> MKFKWDEFFVTGDPLILGAQVSIALSTIAIIFVLTYFKKWKWLWSEWITTVDHKKLGIMYIISAVIMLFRGGVDGLMMRAQLALPNNSFLDSNHYNEIFTTHGTIMIIFMAMPFLIGLINVVVPLQIGARDVAFPYLNNLSFWTFFVGAMLFNISFVIGGSPNAGWTSYMPLASNDMSPGPGENYYLLGLQIAGIGTLMTGINFMVTILKMRTKGMTLMRMPMFTWTTLITMVIIVFAFPVLTVALALLSFDRLFGAHFFTLEAGGMPMLWANLFWIWGHPEVYIVILPAFGIFSEIISSFARKQ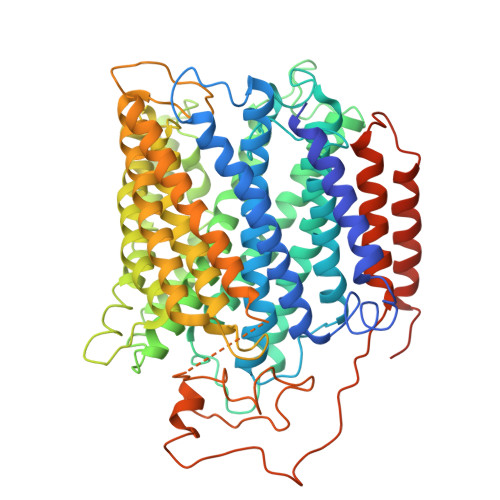LFGYKAMVGSIIAISVLSFLVWTHHFFTMGNSASVNSFFSITTMAISIPTGVKIFNWLFTMYKGRISFTTPMLWALAFIPNFVIGGVTGVMLAMAAADYQYHNTYFLVSHFHYVLIAGTVFACFAGFIFWYPKMFGHKLNERIGKWFFWIFMIGFNICFFPQYFLGLQGMPRRIYTYGPNDGWTTLNFISTVGAFMMGVGFLILCYNIYYSFRYSTREISGDSWGVGRTLDWATSSAIPPHYNFAVLPEVKSQDAFLHMKEEKTELYPESKFKKIHMPSNSGRPFFMSVAFGLAGFGLVFEWYWMGVVGLIGVLLCMVLRSFEYDNGYYISVDEIKETERKISEHHHHHH> MENIQKLIARYPLVEDLVALKETTWFNPGATSLAQGLPYVGLTEQDVNAAHDRLARFAPYLAKAFPQTAAAGGMIESDVVAIP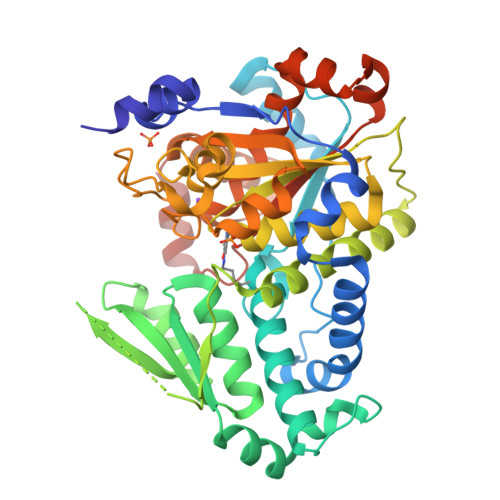AMQKRLEKEYGQTINGEMLLKKDSHLAISGSIKARGGIYEVLTHAEKLALEAGLLTTDDDYSVLLSPEFKQFFSQYSIAVGSAGNLGLSIGIMSACIGFKVTVHMSADARAWKKAKLRSHGVTVVEYEDDYGVAVEQGRKAAQSDPNCFFIDDENSRTLFLGYAVAGQRLKAQFAQQGRVVDASHPLFVYLPCGVGGGPGGVAFGLKLAFGDNVHCFFAEPTHSPCMLLGVYTGLHDAISVQDIGIDNLTAADGLAVGRASGFVGRAMERLLDGLYTLDDQTMYDMLGWLAQEEGIRLEPSALAGMAGPQRICASVAYQQRHGFSQTQLGNATHLVWATGGGMVPEDEMEQYLAKGRLEHHHHHH> LIVLNVSGTRF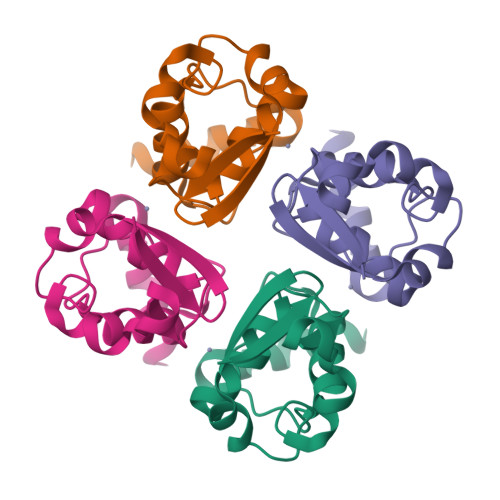QTWQDTLERYPDTLLGSSERDFFYHPETQQYFFDRDPDIFRHILNFYRTGKLHYPRHECISAYDEELAFFGLIPEIIGDCCYEEYKDRRRENAE The Mycobacterium tuberculosis trifunctional enzyme (MtTFE) is an α2β2 tetrameric enzyme in which the α-chain harbors the 2E-enoyl-CoA hydratase (ECH) and 3S-hydroxyacyl-CoA dehydrogenase (HAD) active sites, and the β-chain provides the 3-ketoacyl-CoA thiolase (KAT) active site. Linear, medium-chain and long-chain 2E-enoyl-CoA molecules are the preferred substrates of MtTFE. Mtb is capable of switching its metabolic preference during the latent stage of infection in order to utilize host-derived fatty acids as a source of carbon rather than glucose or glycerol. The Mtb genome encodes an unusually large set of enzymes of the β-oxidation cycle; however, only a single trifunctional enzyme (MtTFE) that catalyzes three of the last four reactions in the β-oxidation cycle is present in Mtb, in contrast to other bacteria such as Escherichia coli, which has two TFEs. Here, 226 fragments were screened in a crystallographic fragment-binding study of MtTFE crystals, resulting in the structures of 16 MtTFE–fragment complexes.

A similar mode of binding is observed for fragment B-H11, which interacts with these two catalytic glutamates using its hydroxyl group. Furthermore, near the CoA-C(ECH/HAD) site, fragments B-H11 and M-72 bind at subsite I1, which perfectly bridges the gap between the bound CoA at the ECH active site and the CoA-C(ECH/HAD) binding site. The distances from the ECH and HAD active sites to the I2 site are approximately 21 and 12 Å, respectively, and the corresponding distance from the KAT active site is approximately 44 Å, when considering the distances between the bridging pyrophosphate O atoms of the CoA molecules bound at these sites. The path is identified by the fragments B-E1, B-H11, M-1, M-49, M-53 and M-72, in addition to the CoA-C(ECH/HAD) molecule.

>[2x]MGSSHHHHHHSQDPNSMPDNTIQWDKDADGIVTLTMDDPSGSTNVMNEAYIESMGKAVDRLVAEKDSITGVVVASAKKTFFAGGDVKTMIQARPEDAGDVFNTVETIKRQLRTLETLGKPVVAAINGAALGGGLEIALACHHRIAADVKGSQLGLPEVTLGLLPGGGGVTRTVRMFGIQNAFVSVLAQGTRFKPAKAKEIGLVDELVATVEELVPAAKAWIKEELKANPDGAGVQPWDKKGYKMPGGTPSSPGLAAILPSFPSNLRKQLKGAPMPAPRAILAAAVEGAQVDFDTASRIESRYFASLVTGQVAKNMMQAFFFDLQAINAGGSRPEGIGKTPIKRIGVLGAGMMGAGIAYVSAKAGYEVVLKDVSLEAAAKGKGYSEKLEAKALERGRTTQERSDALLARITPTADAADFKGVDFVIEAVFENQELKHKVFGEIEDIVEPNAILGSNTSTLPITGLATGVKRQEDFIGIHFFSPVDKMPLVEIIKGEKTSDEALARVFDYTLAIGKTPIVVNDSRGFFTSRVIGTFVNEALAMLGEGVEPASIEQAGSQAGYPAPPLQLSDELNLELMHKIAVATRKGVEDAGGTYQPHPAEAVVEKMIELGRSGRLKGAGFYEYADGKRSGLWPGLRETFKSGSSQPPLQDMIDRMLFAEALETQKCLDEGVLTSTADANIGSIMGIGFPPWTGGSAQFIVGYSGPAGTGKAAFVARARELAAAYGDRFLPPESLLS;>MSEEAFIYEAIRTPRGKQKNGSLHEVKPLSLVVGLIDELRKRHPDLDENLISDVILGCVSPVGDQGGDIARAAVLASGMPVTSGGVQLNRFCASGLEAVNTAAQKVRSGWDDLVLAGGVESMSRVPMGSDGGAMGLDPATNYDVMFVPQSIGADLIATIEGFSREDVDAYALRSQQKAAEAWSGGYFAKSVVPVRDQNGLLILDHDEHMRPDTTKEGLAKLKPAFEGLAALGGFDDVALQKYHWVEKINHVHTGGNSSGIVDGAALVMIGSAAAGKLQGLTPRARIVATATSGADPVIMLTGPTPATRKVLDRAGLTVDDIDLFELNEAFASVVLKFQKDLNIPDEKLNVNGGAIAMGHPLGATGAMILGTMVDELERRNARRALITLCIGGGMGVATIIERV[2x]>GSFVEMVDNLRGKSGQGYYVEMTVGSPPQTLNILVDTGSSNFAVGAAPHPFLHRYYQRQLSSTYRDLRKGVYVPYTQGKWEGELGTDLVSIPHGPNVTVRANIAAITESDKFFINGSNWEGILGLAYAEIARPDDSLEPFFDSLVKQTHVPNLFSLQLCGAGFPLNQSEVLASVGGSMIIGGIDHSLYTGSLWYTPIRREWYYEVIIVRVEINGQDLKMDCKEYNYDKSIVDSGTTNLRLPKKVFEAAVKSIKAASSTEKFPDGFWLGEQLVCWQAGTTPWNIFPVISLYLMGEVTNQSFRITILPQQYLRPVEDVATSQDDCYK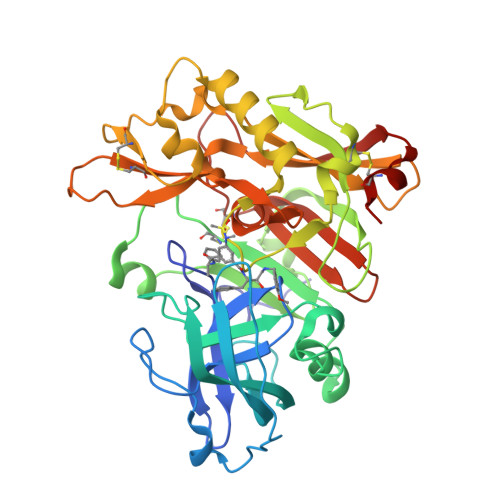FAISQSSTGTVMGAVIMEGFYVVFDRARKRIGFAVSACHVHDEFRTAAVEGPFVTLDMEDCGYN[4x]N-[(S)-[2-(benzoylamino)ethoxy](hydroxy)phosphoryl]-L-glutamic 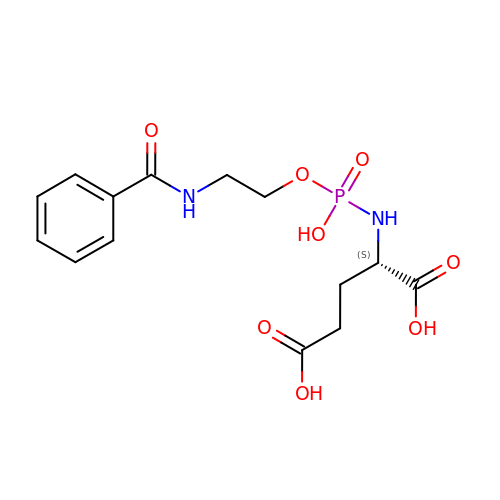acid | C14 H19 N2 O8 P | BBHOFRAKRKNSKD-NSHDSACASA-N>[2x]ASMTGGQQMGAPITAYAQQTRGLLGCIITSLTGRDKNQVEGEVQIVSTATQTFLATCINGV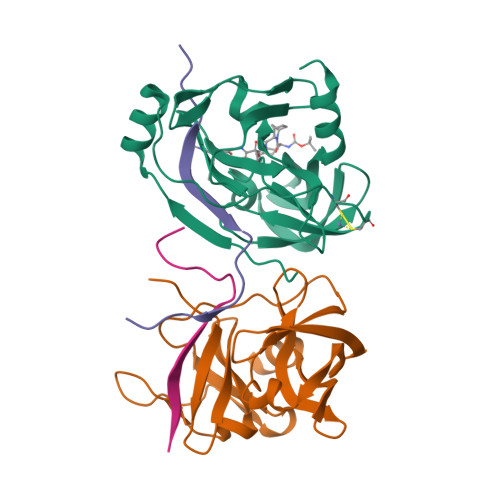CWTVYHGAGTRTIASPKGPVIQMYTNVDQDLVGWPAPQGSRSLTPCTCGSSDLYLVTRHADVIPVRRRGDSRGSLLSPRPISYLKGSSGGPLLCPAGHAVGLFRAAVCTRGVAKAVDFIPVENLETTMRSGSHHHHHH;>[2x]KKGSVVIVGRIVLSGKPAIIPKK>[2x]DDHSELLVNTKSGKVMGTRVPVLSSHISAFLGIPFAEPPVGNMRFRRPEPKKPWSGVWNASTYPNNCQQYVDEQFPGFSGSEMWNPNREMSEDCLYLNIWVPSPRPKSTTVMVWIYGGGFYSGSSTLDVYNGKYLAYTEEVVLVSLSYRVGAFGFLALHGSQEAPGNVGLLDQRMALQWVHDNIQFFGGDPKTVTIFGESAGGASVGMHILSPGSRDLFRRAILQSGSPNCPWASVSVAEGRRRAVELGRNLNCNLNSDEELIHCLREKKPQELIDVEWNVLPFDSIFRFSFVPVIDGEFFPTS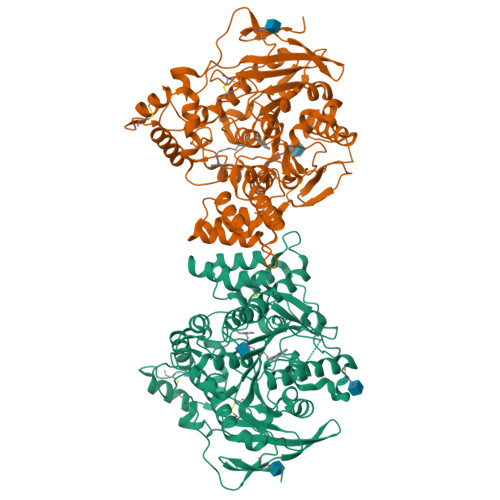LESMLNSGNFKKTQILLGVNKDEGSFFLLYGAPGFSKDSESKISREDFMSGVKLSVPHANDLGLDAVTLQYTDWMDDNNGIKNRDGLDDIVGDHNVICPLMHFVNKYTKFGNGTYLYFFNHRASNLVWPEWMGVIHGYEIEFVFGLPLVKELNYTAEEEALSRRIMHYWATFAKTGNPNEPHSQESKWPLFTTKEQKFIDLNTEPMKVHQRLRVQMCVFWNQFLPKLLNATACDGELSS> MRLERV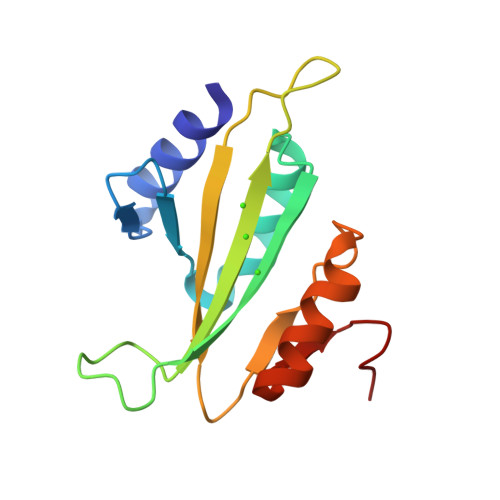LEEARAKGYPIEDNGLGNLWVVLPRERFKEEMAHYKAMGFNFLADIVGLDYLTYPDPRPERFAVVYELVSLPGWKDGDGSRFFVRVYVPEEDPRLPTVTDLWGSANFLEREVYDLFGIVFEGHPDLRK Herein we identify a new glucuronic acid decarboxylase from Micromonospora belonging to the superfamily of short-chain dehydrogenase/reductase enzymes, EvdS6. Biochemical characterization demonstrated that EvdS6 is an NAD+-dependent bifunctional enzyme that produces a mixture of two products, differing in the sugar C-4 oxidation state. At a global level, EvdS6 displays the SDR enzyme architecture and is a dimer with a buried surface area of 2371 Å2 and 2362 Å2 in ligand-free and nucleotide diphosphate-bound states, respectively. In line with the SDR architecture, each protomer consists of two domains: the N-terminal domain consisting of residues V1-Y181 and V219-A242 and the C-terminal domain between residues G182-H218 and G243-L323.

X-ray crystallographic analysis of EvdS6 at 1.51 Å resolution with bound co-factor and TDP demonstrated that the overall geometry of the EvdS6 active site is conserved with other SDR enzymes and enabled studies probing structural determinants for the reductive half of the net neutral catalytic cycle. To better understand the mechanism of catalysis, the commercially available UDP-GlcA was co-crystallized with EvdS6. This resulted in the appearance of new electron density in the active site of each of the two protomers in the dimer. Surprisingly, the electron density at the active site of the first protomer is clearly consistent with TDP rather than UDP, but no density for the glucuronic acid was observed. In the second molecule of the dimer, electron density suggested that the different EvdS6 molecules in the crystal were bound to different species, resulting in a mixed state. Although the density was not readily interpretable, it appears that about 40 to 50% of the molecules in the crystal are likely bound to citrate from the buffer. In terms of the nucleotide diphosphate-binding residues, the TDP binds at the interdomain interface of EvdS6 and has multiple direct interactions with residues of both the N-terminal domain (E128 and N179), and the C-terminal domain (V190, P205, Y207, R214, N249, R273, and H276). The thymine ring of TDP forms a hydrogen bond through its carbonyl oxygen at position two with the backbone amide of Y207; additionally, this aromatic side chain participates in a parallel π-stacking interaction with the thymine ring of TDP. Notably, the binding of TDP is associated with the structuring of a loop between V270 and D284; direct interaction between the side chains of R273 and H276 with TDP facilitates this ordering. In the ligand-free structure, no traceable electron density for residues R273, K274, or G275 or the sidechain of H276 was observed in one of the subunits. The change from disordered to directly interacting with the TDP suggests that this flexible loop could be involved in binding and coordinating the substrate in the active site.

>[2x]MGSSHHHHHHSSGLVPRGSVPRVFVAGGAGFIGSHYVRELVAGAYAGWQGCEVTVLDSLTYAGNLANLAGVRDAVTFVRGDICDGRLLAEVLPGHDVVLNFAAETHVDRSIADSAEFLRTNVQGVQSLMQACLTAGVPTIVQVSTDEVYGSIEAGSWSEDAPLAPNSPYAAAKAGGDLIALAYARTYGLPVRITRCGNNYGPYQFPEKVIPLFLTRLMDGRSVPLYGDGRNVRDWIHVADHCRGIQTVVERGASGEVYHIAGTAELTNLELTQHLLDAVGGSWDAVERVPDRKGHDRRYSLSDAKLRALGYAPRVPFADGLAETVAWYRANRHWWEPLRKQLDAVPHD>VRRDRAPPERGGAGTSQDGTSKNWFKITIPYGRKYDKAWLLSMIQSKCSVPFTPIEFHYENTRAQFFVEDASTASALKAVNYKILDRENRRISIIINSSAPPHTILNELKPEQVEQLKLIMSKRYDGSQQALDLKGLRSDPDLVAQNIDVVLNRRSCMAATLRIIEENIPELLSLNLSN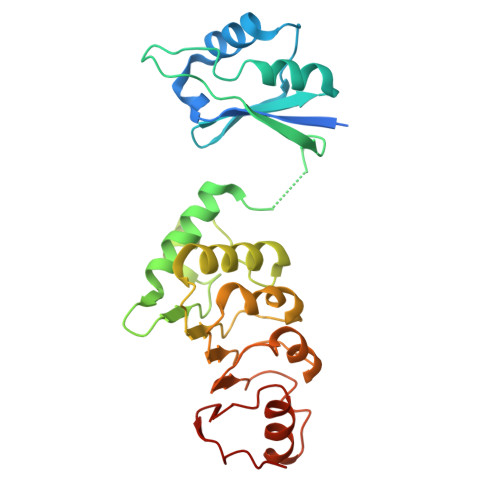NRLYRLDDMSSIVQKAPNLKILNLSGNELKSERELDKIKGLKLEELWLDGNSLCDTFRDQSTYISAIRERFPKLLRLDGHELPPPIAF[4x]> GSTLTYPFHDWSQELSPRYAQLRASDAPVCPVVSEGTGDPLWLVTRYATAVKLLEDSRFSSEAAQASGAPRQEPVELRAPGTRGDAIAMLREAGLRSVLADGLGPRAVRRHQGWINDLAETLMSELASREGTFDLAADFVEPLSSALVSRTLLGELSADERDLLAHCADTGLRFCGVTHEEQVHAFTQMHEFFLEHARRLAGT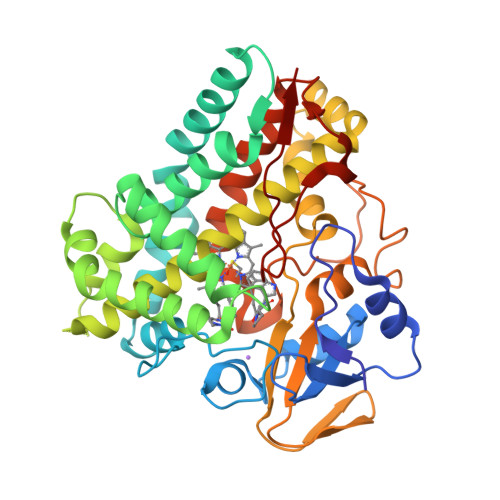PGEHLLKLIAEAPVDQGPLSDEALAEAGSLLVVAGFPTSSGFLCGALLTLLRHPDAVQELHAHPERVPSAVEELLRYTPLATGSAKRMATEDLEIDGVRIKAGEVVMVSLEAVNHDPDAFEDPDVFRPGREGPMHFGFGRGRHFCPGNRLARCVIEATVRAVARRPGLRLAVAPEEISWHEGLFFRRPRAIPATW>[2x]NDMKLAPPT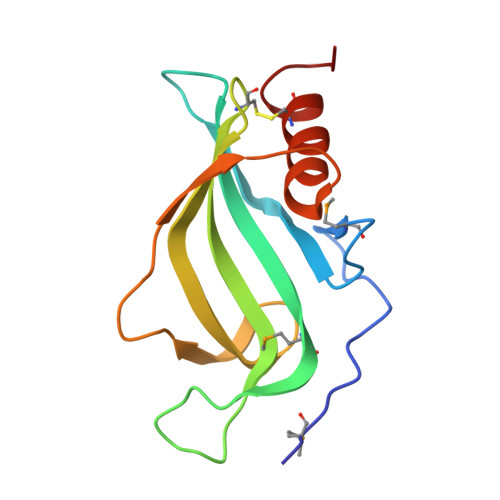DVRSGYIRMVKNVNYYIDSESIWVDNQEPQIVHFDAVVNMDRGLYVYPEPKRYARSVRQYKILNCANYHLTQVRTDFYDEFWGQGLRAAPKKQKKHTLSLTPDTTLYNAAQIICANYGKAFSV> MLAYQGTQIKEKRDEDAGFDLCVP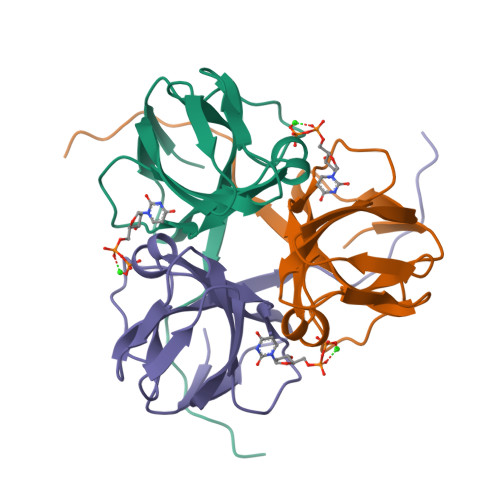YDIMIPVSDTKIIPTDVKIQVPPNSFGWVTGKSSMAKQGLLINGGIIDEGYTGEIQVICTNIGKSNIKLIEGQKFAQLIILQHHSNSRQPWDENKISQRGDKGFGSTGVF> SNAIAQQWAIFRDKYFHPNGRIIDTGNSGESHSEGQGYGMLFSAAAGDQAAFEVIWVWARTNLQHKDDALFSWRYLDGHKPPVADKNNATDGDLLIALALAWAGKRWKRADYIQDAMNIYGDVLKLMTKSVGPYT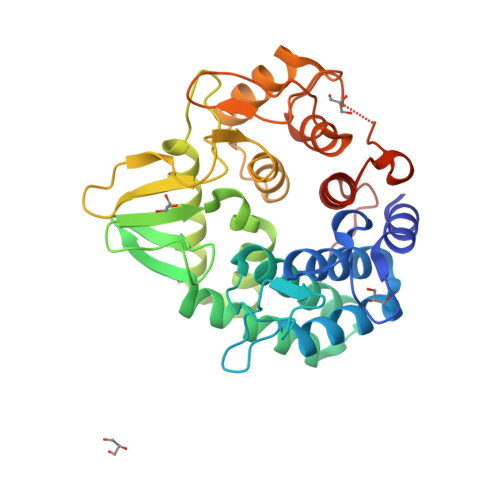VLLPGAVGFLTKDTVTLNLSYYVMPSLMQAFALTGDAKWTKVMGDGLQIIAKGRFGEWKLPPDWLSINLHTNAFSIAKGWPPRFSYDAIRVPLYLSWAHMLTPELLADFSRFWNHYGASALPGWVDLTNGARSPYNAPPGYLAVASCTGLASAGELPTLDHAPDYYSAALTMLAYIARNQADLYFA Plectasin consists of 40 amino acids and shows well-defined secondary structural elements in form of an α-helix (M13-S21) and an antiparallel β-sheet (G28-A31; V36-C39). The structure of plectasin is stabilized by three disulfide bridges (C4-C30; C15-C37; C19-C39), which is typical for this type of defensins and leads to high conformational stability. Plectasin contains a cysteine-stabilised α-helix-β-sheet structure, which remains intact upon fibril formation. We have determined the structure, kinetics, and functionality associated with the pH-responsive self-assembly of the enhanced plectasin variant PPI42 into helical protein fibrils.

In our negative stain EM measurement, we observed a small portion of fibrils existing as single protofilaments. In order to investigate whether there are structural rearrangements upon formation of the mature fibril, we analyzed the 3.4 Å resolution structure of PPI42 forming the single protofilament obtained by cryo-EM. The structure of the protofilament was determined using the structure of the mature fibril. PPI42 monomers show a very similar arrangement in the protofilament compared to the mature fibril (all-atom RMSD: 0.727 Å). The PPI42 protofilament forms a straight right-handed helical structure having an axial rise of 3.76 Å and a helical twist of 156.5° between two monomers. These helical parameters are very close to the seven monomers of the asymmetric unit in the mature fibril (average axial rise of 3.75 ± 0.15 Å and an average twist of 156.48 ± 2.25° between two consecutive monomers, see above). Small variations in axial rise and twist between the monomers in the mature fibril result from the curvature of the protofilament, which is then stabilized by the interaction with a second protofilament. A comparison between the cryo-EM structure of the mature fibril and of the isolated protofilament showed high similarity, indicating that protofilaments form prior to the supramolecular assembly into a curved mature fibril without additional structural rearrangement. We observed frayed fibril termini and a small number of single protofilaments (black arrows), suggesting that the protofilaments formed first and then assembled into the mature fibrils.

>GFGCNGPWSEDDMKCHNHCKSIKGYKGGYCAKGGFLCKCY[25x]> MDTEVYES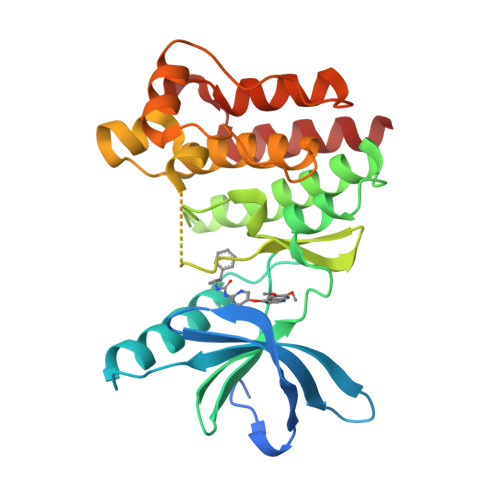PYADPEEIRPKEVYLDRKLLTLEDKELGSGNFGTVKKGYYQMKKVVKTVAVKILKNEANDPALKDELLAEANVMQQLDNPYIVRMIGICEAESWMLVMEMAELGPLNKYLQQNRHVKDKNIIELVHQVSMGMKYLEESNFVHRDLAARNVLLVTQHYAKISDFGLSKALRADENYYKAQTHGKWPVKWYAPECINYYKFSSKSDVWSFGVLMWEAFSYGQKPYRGMKGSEVTAMLEKGERMGCPAGCPREMYDLMNLCWTYDVENRPGFAAVELRLRNYYYDVVN>[4x]MPALKKQRIDLRLTDDDKSIIEEAAAISNQTITQFVVASASERAAEVIEQHRRMVLNEQSWSLVMEAITQPPAPNDRLKRAAKRLQTR;>MEQQLTIEMIADAFSYDITGFDCGEEALNTFLKEHLKRQHDGQILRGYALVSGDTVPRL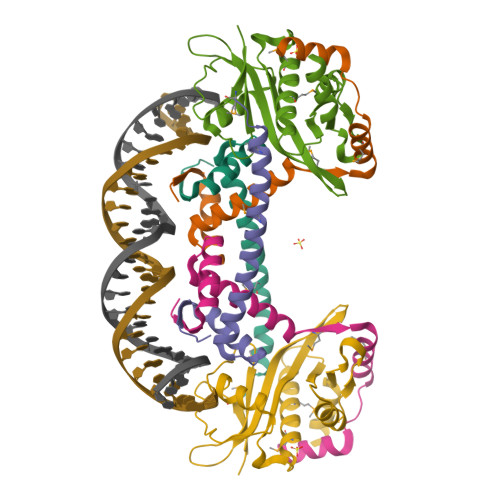LGYYTLSGSCFERGMLPSKTQQKKIPYQNAPSVTLGRLAIDKSVQGQGWGEMLVAHVMRVVWGASKAVGIYGLFVEALNEKAKAFYLRLGFIQLVDENSNLLFYPTKSIEQLFTDDES[2x]> GGSYGYDAFFRGAAEVLNGSNIQLPHLPENEEQKEGKVYQLHSVRFPPQVRRLGANYFFRRQRAVPLTYYHHLVEAKPASEGSAPDGV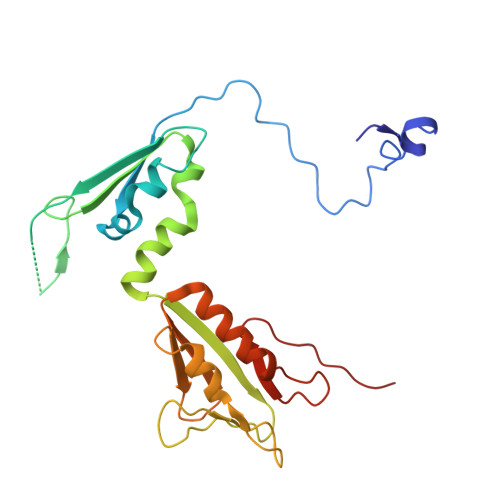HAQTGRGQALCFVASANPGYLQSKELENAVFESTRGFACQLILEGRGVKAYFDPEWPNLMVRLGVGVKPLALRRLAEQYATRAKIFVDKRGLLLTVHGYDKCAVGTLAMSLFNHLQANPYTMKGAHVAMHPIKKKVTR> GPLGSAAAVESVVSDETLSSNPLLQDFDFPPFDSVDASHVRPGIRALLQHLEAELEELEKSVEPTWPKLVEPLEKIVDRLTVVWGMINHLKAVKDTPELRAAIEDVQPEKVKFQLRLGQSKPIYNAFKAIRESPDWSSLSEARQRLVEAQIKEAVLIGIALDDEKREEFNKIEQELEKLSHKFSENVLDATKKFEKLITDKKEIEGLPPSALGLFAQAAVSKGHENATAENGPWIITLDAPSYL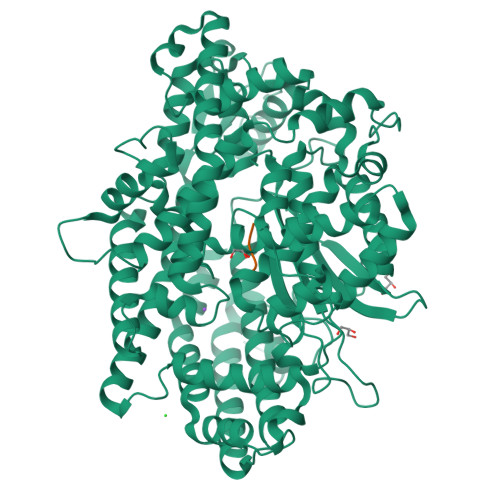PVMQHAKNRALREEVYRAYLSRASSGDLDNTAIIDQILKLRLEKAKLLGYNNYAEVSMAMKMATVEKAAELLEKLRSASWDAAVQDMEDLKSFAKNQGAAESDSMTHWDTTFWSERLRESKYDINEEELRPYFSLPKVMDGLFSLAKTLFGIDIEPADGLAPVWNNDVRFYRVKDSSGNPIAYFYFDPYSRPSEKRGGAWMDEVVSRSRVMAQKGSSVRLPVAHMVCNQTPPVGDKPSLMTFREVETVFHQFGHALQHMLTKQDEGLVAGIRNIEWDAVELPSQFMENWCYHRDTLMSIAKHYETGETLPEEVYKKLLAARTFRAGSFSLRQLKFASVDLELHTKYVPGGPESIYDVDQRVSVKTQVIPPLPEDRFLCSFSHIFAGGYAAGYYSYKWAEVLSADAFSAFEDAGLDDIKAVKETGQRFRNTILALGGGKAPLKVFVEFRGREPSPEPLLRHNGLLAASASA;> AAAA> GPLLEMILITGSNGQLGTELRYLLDERGVDYVAVDVAEMDITNEDKVEAVFAQVKPTLVYHCAAYTAVDAAEDEGKALNEAINVTGSENIAKACGKYGATLVYISTDYVFDGNKPVGQEWVETDHPDPKTEYGRTKRLGELAVERYAEHFYIIRTAWVFGNYGKNFVFTMEQLAENHSRLTVVNDQHGRPTWTRTLAEFMCYLTENQKAFGYYHLSNDAKEDTTWYDFAKEILKDKAVEVVPVDSSAFPAKAKRPLNSTMN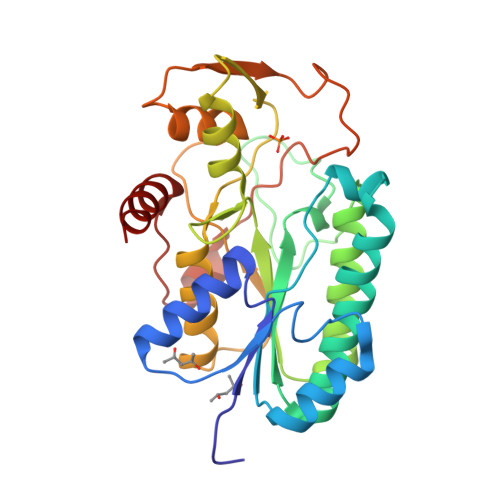LDKAKATGFVIPTWQEALKAFYQQGLKK>MKASPHRPTKALIHLGAIRQNIQQMGAHIPQGTLKLAVVKANAYGHGAVAVAKAIQDDVDGFCVSNIDEAIELRQAGLSKPILILGVSEIEAVALAKEYDFTLTVAGLEWIQALLDKEVDLTGLTVHLKIDSGMGRIGFREASEVEQAQDLLQQHGVCVEGIFTHFATADEESDDYFNAQLERFKTILASMKEVPELVHASNSATTLWHVETIFNAVRMGDAMYGLNPSGAVLDLPYDLIPALTLESALVHVKTVPAGA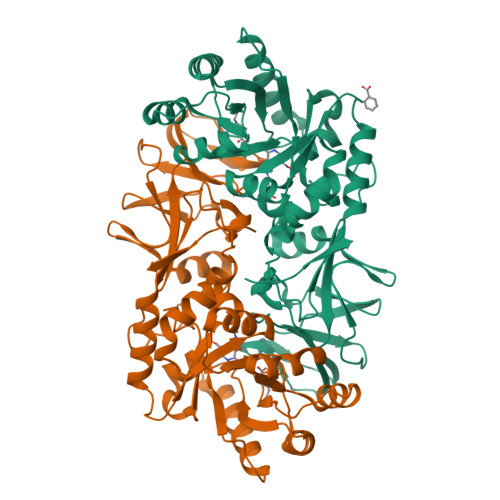CMGYGATYQADSEQVIATVPIGYADGWTRDMQNFSVLVDGQACPIVGRVSMDQITIRLPKLYPLGTKVTLIGSNGDKEITATQVATYRVTINYEVVCLLSDRIPREYY[2x]> MMTLNRKCVVIHNGSHRTVAGFSNVELPQCIIPSSYIKRTDEGGEAEFIFGTYNMIDAAAEKRNGDEVYTLVDSQGLPYNWDALEMQWRYLYDTQLKVSPEELPLVITMPATNGKPDMA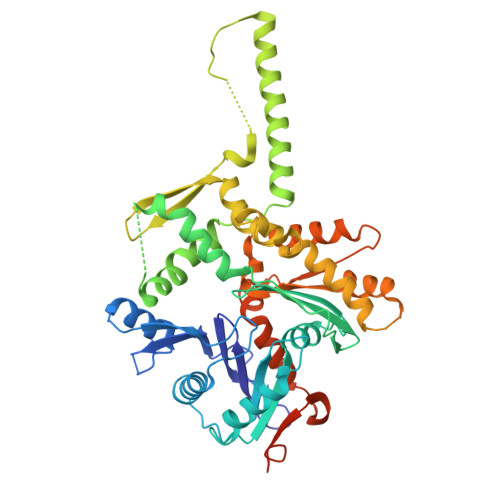ILERYYELAFDKLNVPVFQIVIEPLAIALSMGKSSAFVIDIGASGCNVTPIIDGIVVKNAVVRSKFGGDFLDFQVHERLAPLIKEENDMENMADEQKRSTDVWYEASTWIQQFKSTMLQVSEKDLFELERYYKEQADIYAKQQEQLKQMDQQLQYTALTGSPNNPLVQKKNFLFKPLNKTLTLDLKECYQFAEYLFKPQLISDKFSPEDGLGPLMAKSVKKAGASINSMKANTSTNPNGLGTSHINTNVGDNNSTASSSNISPEQVYSLLLTNVIITGSTSLIEGMEQRIIKELSIRFPQYKLTTFANQVMMDRKIQGWLGALTMANLPSWSLGKWYSKEDYETLKRDRKQSQATNATNLVPRGSHHHHHH>MSRLVVVSNRIAPPDEHAASAGGLAVGILGALKAAGGLWFGWSGETGNEDQPLKKVKKGNITWASFNLSEQDLDEYYNQFSNAVLWPAFHYRLDLVQFQRPAWDGYLRVNALLADKLLPLLQDDDIIWIHDYHLLPFAHELRKRGVNNRIGFFLHIPFPTPEIFNALPTYDTLLEQLCDYDLLGFQTENDRLAFLDCLSNLTRVTTRSAKSHTAWGKAFRTEVYPIGIEPKEIAKQAAGPLPPKLAQLKAELKNVQNIFSVERLDYSKGLPERFLAYEALLEKYPQHHGKIRYTQIAPTSRGDVQAYQDIRHQLENEAGRINGKYGQLGWTPLYYLNQHFDRKLLMKIFRYSDVGLVTPLRDGMNLVAKEYVAAQDPANPGVLVLSQFAGAANELTSALIVNPYDRDEVAAALDRALTMSLAERISRHAEMLDVIVKNDINHWQECFISDLKQIVPRSAESQQRDKV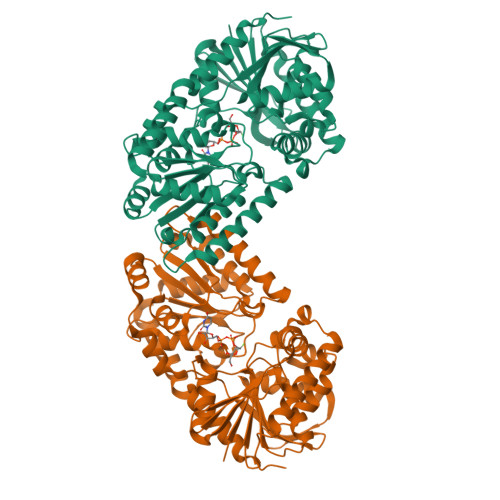ATFPKLALEHHHHHH[2x]> MGNITADNSSMSCTIDHTIHQTLAPVVYVTVLVVGFPANCLSLYFGYLQIKARNELGVYLCNLTVADLFYICSLPFWLQYVLQHDNWSHGDLSCQVCGILLYENIYISVGFLCCISVDRYLAVAHPFRFHQFRTLKAAVGVSVVIWAKELLTSIYFLMHEEVIEDENQHRVCFEHYPIQAWQRAINYYRFLVGFLFPICLLLASYQGILRAVRRSHGTQKSRKDQIQRLVLSTVVIFLACFLPYHVLLLVRSVWEASC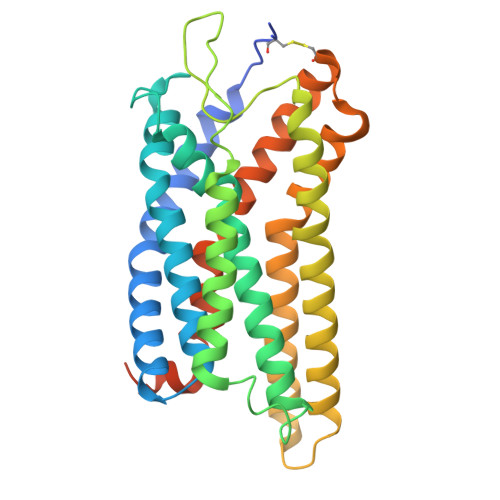DFAKGVFNAYHFSLLLTSFNCVADPVLYCFVSETTHRDLARLRGACLAFLTCSRTGRAREA> LYIQWL

Here, we identify an evolutionarily conserved hexapeptide sequence as the major aggregation-prone region (APR) of gastrointestinal peptides of the glucagon family: xFxxWL. We determine nine polymorphic crystal structures of the APR segments of glucagon-like peptides 1 and 2, and exendin and its derivatives. We propose that the pH-dependent changes of the protonation states of glutamate/aspartate residues of APRs initiate switching between the amyloid and the folded, monomeric forms of the hormones. Our results highlight the dual role of short aggregation core motifs in reversible amyloid formation and receptor binding.

APRTc5b does not contain gatekeeper residues and is thus capable of amyloid formation over a broad range of pH (2 < pH < 11). Four polymorphic crystal forms were grown from solutions of APRTc5b. Although the chains in polymorph B are also arranged according to the class 8 topology, different interactions stabilize the interfaces. While in polymorphs A and C Tyr, Gln, and Trp form H-bonds at the β-sheet/β-sheet interface with each other, this arrangement allows their interactions with water molecules and chain termini. Polymorphs formed in pure aqueous solution are laterally displaced, as the side chains of Tyr, Glu, and Gln rather form H-bonds with the surrounding water molecules.> MGKNVVVLGTQWGDEGKGKVVDLLTERAKYVVRYQGGHNAGHTLVINGEKTVLHLIPSGILRENVISIIGNGVVLAPDALMKEMTELEARGVPVRERLLLSEACPLILPYHVALDNAREKARGAKAIGTTGRGIGPAYEDKVARRGLRVSDLFNKETFAIKLKEIVEYHNFQLVHYYKEAAVDYQKVLDDVLAIADILTAMVVDVSELLDNARKQGELIMFEGAQGTLLDIDHGTYPYVTSSNTTAGGVATGSGLGP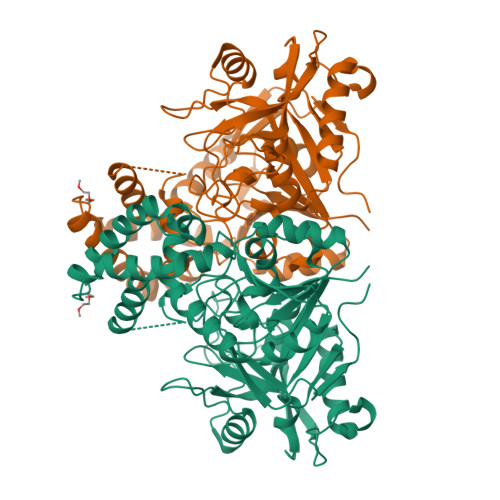RYVDYVLGIVKAYSTRVGAGPFPTELNDETGEFLRKQGNEYGATTGRSRRTGWLDIVAVRRAVQINSLSGFCMTKLDVLDGLKEVKLCVGYRMPDGREVDTTPLAAEGWEGIEPIYETMPGWSETTFGVKEHSKLPQAALNYIQRVEELTGVPIDIISTGPDRDETMILRDPFDA> MIPRGLSEAKPAT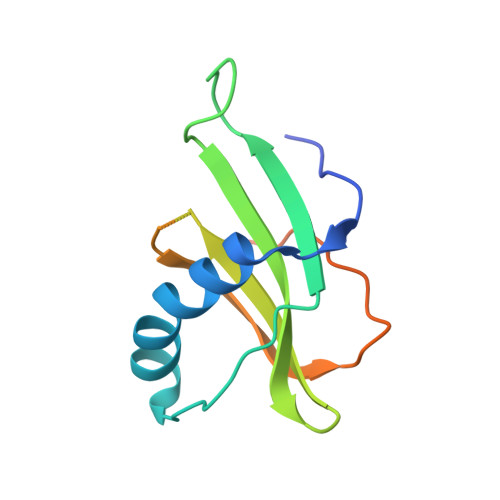PEIQEIVDKVKPQLEEKTNETYGKLEAVQYKTQVLDTYRYILASTNYYIKVRAGDNKYMHLKVFNGPEQKLISEEDLADRVLTGYQVDKNKDDELTGFENLYFQSLERYLEHHHHHH>[2x]GPLGSEDDLYRQSLEIISRYLREQATG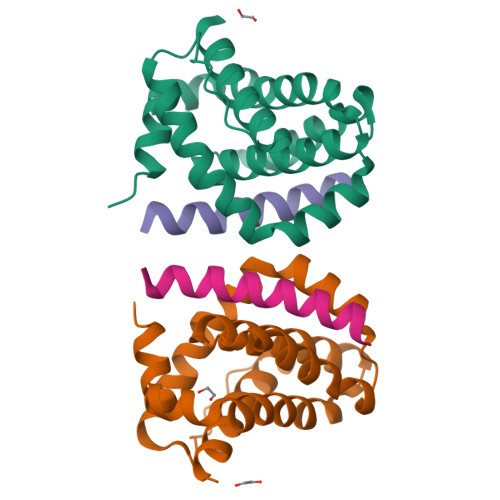SKDSKPLGEAGAAGRRALETLRRVGDGVQRNHETAFQGMLRKLDIKNEDDVKSLSRVMIHVFSDGVTNWGRIVTLISFGAFVAKHLKTINQESCIEPLAESITDVLVRTKRDWLVKQRGWDGFVEFFHVEDLEGG;>DMRPEIRIAQELRRXGDEFNATYARR[2x]>[4x]HHHHHHSSGENLYFQGMQTDSNPHDLAVAGILEQLEGCLRASDSTGAAQLFEPDGYWRDLVLFTWNLKTLEGREQIAAMLAAQLGAVQPVSIRIADGEHAVEAGGVLQSWITVETNVARGVGFIRIRDGKIWTLLTTMSELKGFEEAKGGRRPMGAEHGARTDRSSWLEQREQEAKELGYARQPYCVIIGGGQGGIALGARLRQLNVPTIIIEKNARPGDSWRKRYKSLCLHDPVWYDHMPYIPFPDNWPVFTPKDKVGDWLEMYTKVMELNYWGSTSCESASFDAASGEWTVQVLRDGQPVTLKPKQLVLATGMSGKANMPKFKGMDVFQGEQQHSSQHPGPDAYAGKKVVVVGANNSAHDICAALWEAGVDVTMVQRSSTHIVKSDSLMDLALGDLYSERALAAGMTTNKADLTFASIPYKILANFQKPVFKAIRERDADFYARLEERGFMLDFGDDDSGLFMKYLRRGSGYYIDVGASELVAEGKIKLKSGVGVQELKSHSIVLSDGTELPADLVVYATGYGSMNGWAADLISPEVANKVGKVWGLGSATTKDPGPWEGEQRNMWKPTQQQALWFHGGNLHQSRHYSQYLSLQLKARMEGLNTPVYGQQEVHHLS

In this study, we report the first crystal structure and biochemical characterization of a type II FMO from the Antarctic bacterium Janthinobacterium svalbardensis. The enzyme retains most of its activity at low temperatures and catalyzes the monooxygenation of sulfide compounds as well as linear and cyclic ketones with cofactor promiscuity, enabling low-temperature applications of BVMOs. Type II FMOs are also single-component enzymes and use NAD(P)H and FAD. Among the diverse groups of flavin-containing monooxygenases, type II flavin-containing monooxygenases have been receiving increasing attention as they display cofactor flexibility, accepting both NADH and NADPH.23−25 This feature makes the type II FMO subclass appealing for whole-cell biocatalysis as they can use both cofactors available in the cell.

In the crystal structure, JsFMO appears as a homodimer, with an extended dimerization interface of approximately 2300 Å2, consistent with results from size exclusion chromatography. Four protomers forming two dimers are present in the asymmetric unit. Each protomer appears to be divided into two domains; an N-terminal domain with a SnoaL-like fold and a C-terminal monooxygenase domain (MoD), bearing two typical Rossman folds for FAD and NAD(P)H binding. The two domains are in contact with each other and are connected by a long loop (residues 126–150), a short alpha helix (residues 151–161), and a short unstructured “spacer” (residues 162–170). Contrary to what was initially proposed, the N-terminal domain seems unlikely to be involved in the Baeyer–Villiger monooxygenase activity since it is quite distant from the active site of the MoD. While chains A, B, and C are highly similar with respect to the protein and the cofactor, chain D shows some differences. First, the isoalloxazine ring and part of the ribityl chain of the FAD appear rotated by approximately 15°; furthermore, the isoalloxazine ring appears to slide slightly forward, reducing the space between the flavin and the side-chain of His-216. Another notable difference is the movement of the NADPH-binding domain that, in chain D, seems to tilt toward the active site. No NADP+ is present in the crystal structure, so the movement of this domain must be due to its intrinsic flexibility. The active site of the enzyme is accessible only through a tunnel, with Tyr-458, Asp-217, and His-216 as catalytic residues, a combination not observed before in FMOs and BVMOs.>ASAKELACQEITVPLCKGIGYQYTYMPNQFNHDTQDEAGLEVHQFWPLVEIQCSPD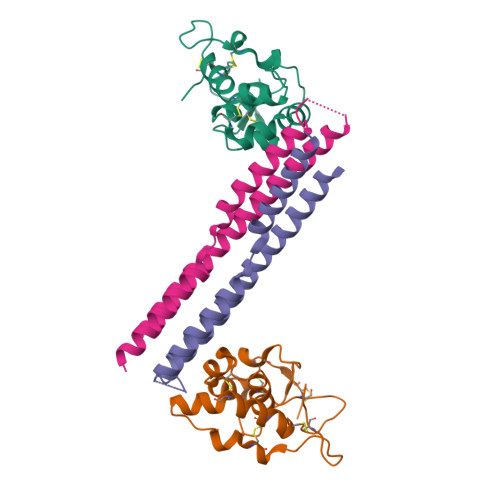LKFFLCSMYTPICLEDYKKPLPPCRSVCERAKAGCAPLMRQYGFAWPDRMRCDRLPEQGNPDTLCMDHHHHHH[2x];>GGVSFSEVMGKQKDEQAREQLKEGMIKIEEQGKKLSETRTQEELQKYVAAVATFALQAGFLGPNLEERRGFNRRGKEEIGKISGEVYLKLLDLKKAVRAKEKKGLDILNMVGEIKGTLERVYA[2x]> MFKSLALVALATISPSALCAPITSRDIPFGQVITTCTTPNTVALTFDDGPSSYTPQLLDLLSEYKVRATFFVLGEASQSNPQIIQRIRQEGHQ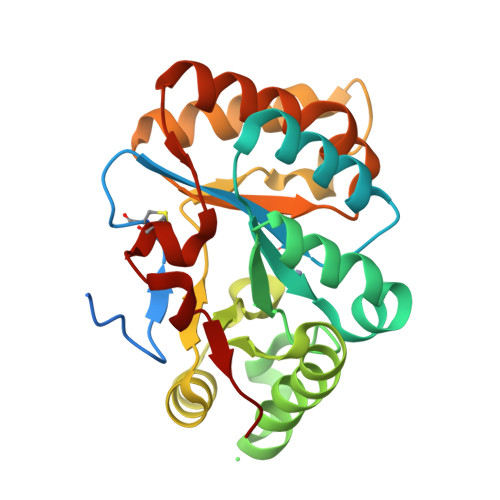VGSHTYDHTSLPTLSYDQIVQEMTSLESVLQSTMGDIPTYMRPPYFDVNDLTLQVMSDLGYHVVTASIDTKDYNHNSPDLISQSYDKFVTELNNGGNLCLAHDTKEQTVVTLAKMMLDETKSRGLTVTTVGDCLGDPEASWYRSSR> ASDHQTQAGKPQSLNPKIIIFEQENFQGHSHELNGPCPNLKETGVEKAGSVLVQAGPWVGYEQANCKGEQFVFEKGEYPRWDSWTSSRRTDSLSSLRPIKVDSQEHKIILYENPNFTGKKMEIIDDDVPSFHAHGYQEKVSSVRVQSGT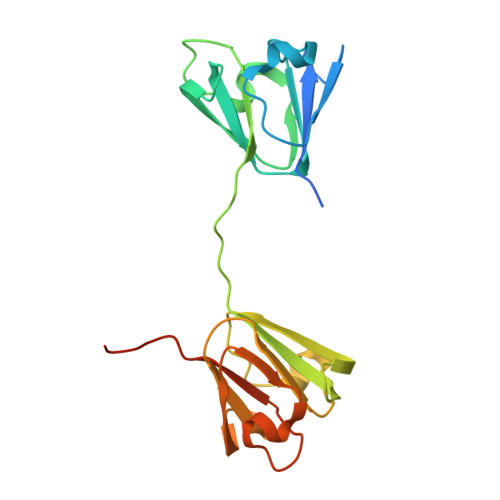WVGYQYPGYRGLQYLLEKGDYKDSSDFGAPHPQVQSVRRIRDMQWHQRGAFHPSN>[3x]MSAKVYFHETFENRDKWIDSTSSGKALGPFKIVSGKWYGDANNKGLQTSEDNKFYIAAAKLDEEFSNKDKNLIVQYNLKFEQGIDCGGGYIKLLPKKSIESEEKFTPESE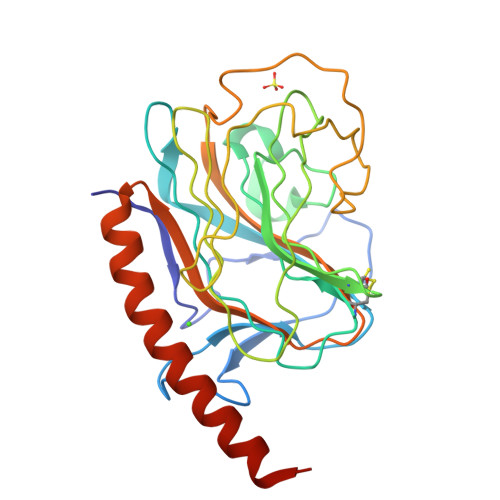YNIMFGPDVCGGSKRTHVIMNYKGKNNLIRKEIKCESDDISHLYTLIIRPNNTYVVKIDGVEKQEGKFDEDWDMLAPKEIDDGSGIANPDYVYDPELYKYDSFAYIGIDVWQVKAGTIYDDILITDDIEEAEKEAKVILERNAAEKKMRDEIKEAENGHHHHHH> ASMERFLSVYDEVQAFLLDQLQSKYEIDPNRARYLRIMMDTTCLGGKYFRGMTVVNVAEGFLAVTQHDEATKERI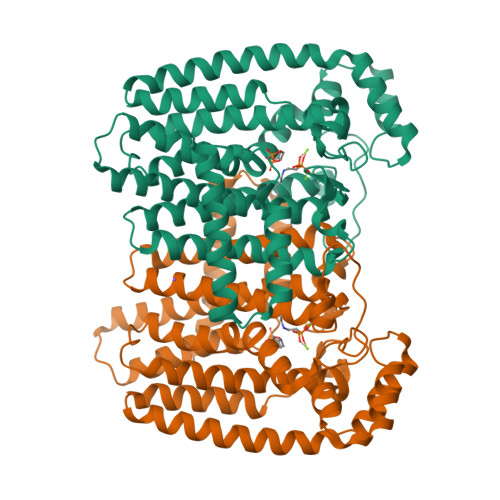LHDACVGGWMIEFLQAHYLVEDDIMDGSVMRRGKPCWYRFPGVTTQCAINDGIILKSWTQIMAWHYFADRPFLKDLLCLFQKVDYATAVGQMYDVTSMCDSNKLDPEVAQPMTTDFAEFTPAIYKRIVKYKTTFYTYLLPLVMGLFVSEAAASVEMNLVERVAHLIGEYFQVQDDVMDCFTPPEQLGKVGTDIEDAKCSWLAVTFLGKANAAQVAEFKANYGDKDPAKVAVVKRLYSEANLQADFAAYEAEVVREVESLIEQLKVKSPTFAESVAVVWEKTHKRKK>[2x]ISEFARAQLSEAMTLASGLKTKVSDIFSQDGSCPANTAATAGIEKDTDINGKYVAKVTTGGTAAA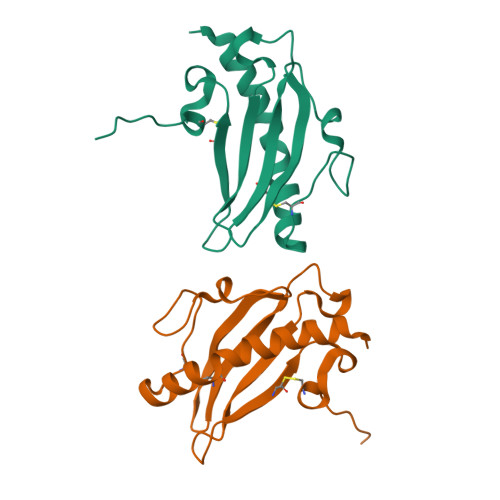SGGCTIVATMKASDVATPLRGKTLTLTLGNADKGSYTWACTSNADNKYLPKTCQTATTTTP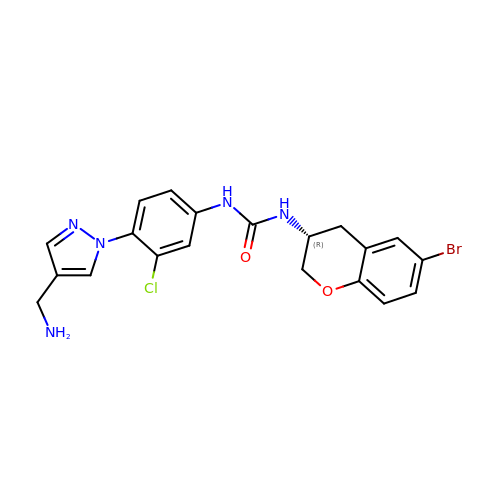1-[4-[4-(aminomethyl)pyrazol-1-yl]-3-chloranyl-phenyl]-3-[(3~{R})-6-bromanyl-3,4-dihydro-2~{H}-chromen-3-yl]urea | C20 H19 Br Cl N5 O2 | DHIWXRKMNHPISE-MRXNPFEDSA-N>MADKAKPAKAANRTPPKSPGDPSKDRAAKRLSLESEGAGEGAAASPELSALEEAFRRFAVHGDARATGREMHGKNWSKLCKDCQVIDGRNVTVTDVDIVFSKIKGKSCRTITFEQFQEALEELAKKRFKDKSSEEAVREVHRLIEGKAPIISGVTKAISSPTVSRLTDTTKFTGSHKERFDPSGKGKGKAGRVDLVDESGYVSGYKHA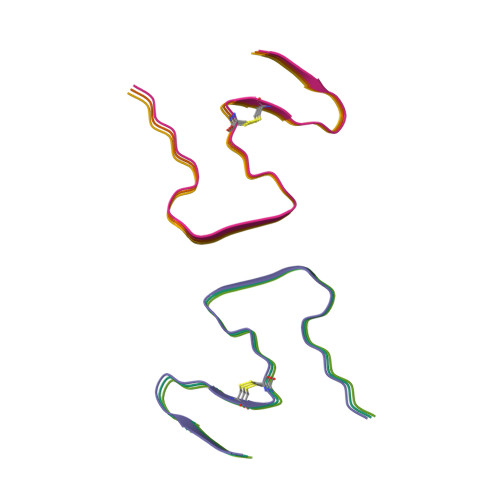GTYDQKVQGGK[6x]> GAMGSF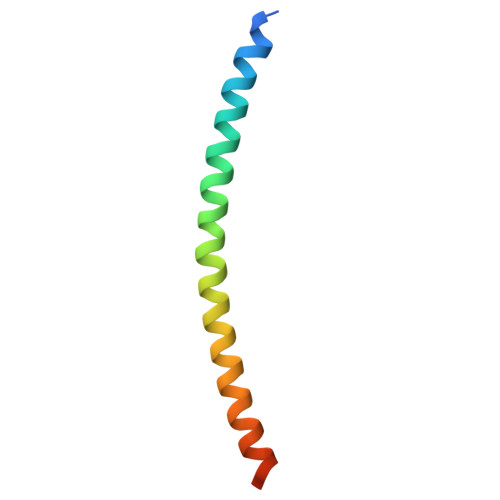NSSINNIHEMEIQLKDALEKNQQWLVYDQQREVYVKGLLAKIFELEKKTETAAHSLP> RSMGDSKRVFG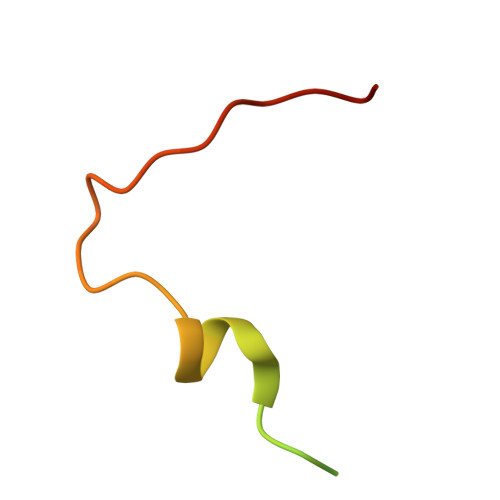ERRRNDSYTEEEPEWFSAGPTSQSETIELTGFD>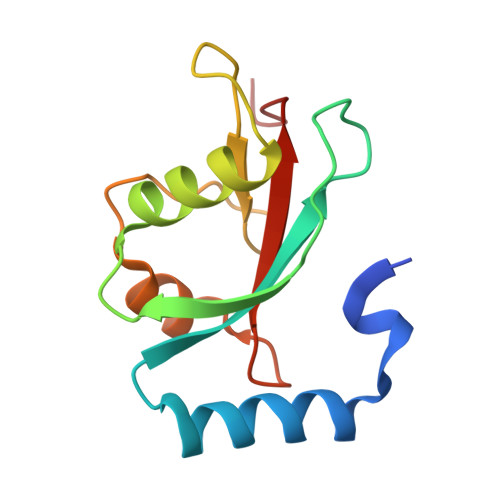 GSMKSTFKSEYPFEKRKAESERIADRFPNRIPVICEKAEKSDIPEIDKRKYLVPADLTVGQFVYVIRKRIMLPPEKAIFIFVNDTLPPTAALMSAIYQEHKDKDGFLYVTYSGENTFG methyl 3-amino-5-(3,5-dimethyl-1,2-oxazol-4-yl)benzoate | C13 H14 N2 O3 | 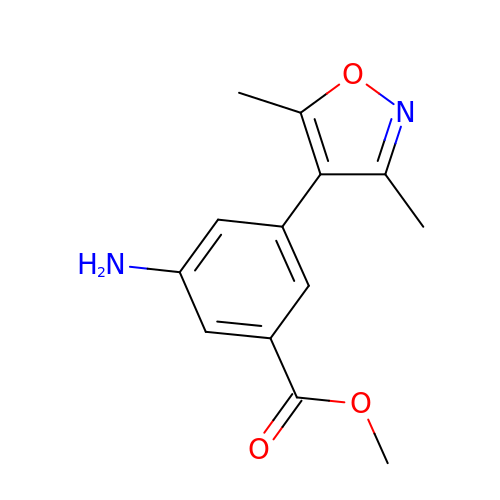CEGDWRFGPGOTIM-UHFFFAOYSA-N2-deoxy-alpha-D-arabino-hexopyranose | C6 H12 O5 | 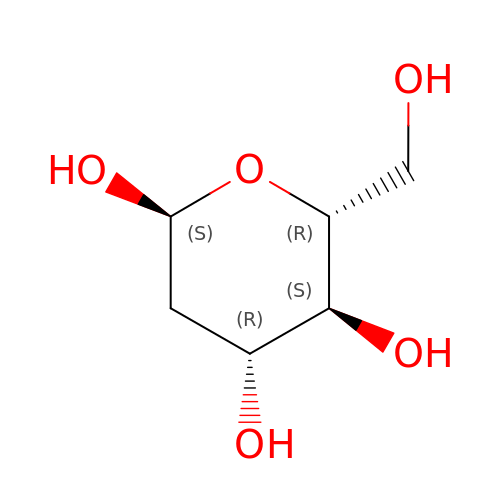PMMURAAUARKVCB-ZXXMMSQZSA-N> MEKETGPEVDDSKVTYDTIQSKVLKAVIDQAFPRVKEYSLNGHTLPGQVQQFNQVFINNHRITPEVTYKKINETTAEYLMKLRDDAHLINAEMTVRLQVVDNQLHFDVTKIVNHNQVTPGQKIDDESKLLSSISFLGNALVSVSSDQTGAKFDGATMSNNTHVSGDDHIDVTNPMKDLAKGYMYGFVSTDKLAAGVWSNSQNSYGGGSNDWTRLTAYKETVGNANYVGIHSSEWQWEKAYKGIVFPEYTKELPSAKVVITEDANADKNVDWQDGAIAYRSIMNNPQGWEKVKDITAYRIAMNFGSQAQNPFLMTLDGIKKINLHTDGLGQGVLLKGYGSEGHDSGHLNYADIGKRIGGVEDFKTLIEKAKKYGAHLGIHVNASETYPESKYFNEKILRKNPDGSYSYGWNWLDQGINIDAAYDLAHGRLARWEDLKKKLGDGLDFIYVDVWGNGQSGDNGAWATHVLAKEINKQGWRFAIEWGHGGEYDSTFHHWAADLTYGGYTNKGINSAITRFIRNHQKDAWVGDYRSYGGAANYPLLGGYSMKDFEGWQGRSDYNGYVTNLFAHDVMTKYFQHFTVSKWENGTPVTMTDNGSTYKWTPEMRVELVDADNNKVVVTRKSNDVNSPQYRERTVTLNGRVIQDGSAYLTPWNWDANGKKLSTDKEKMYYFNTQAGATTWTLPSDWAKSKVYLYKLTDQGKTEEQELTVKDGKITLDLLANQPYVLYRSKQTNPEMSWSEGMHIYDQGFNSGTLKHWTISGDASKAEIVKSQGANDMLRIQGNKEKVSLTQKLTGLKPNTKYAVYVGVDNRSNAKASITVNTGEKEVTTYTNKSLALNYVKAYAHNTRRNNATVDDTSYFQNMYAFFTTGADVSNVTLTLSREAGDEATYFDEIRTFENNSSMYGDKHDTGKGTFKQDFENVAQGIFPFVVGGVEGVEDNRTH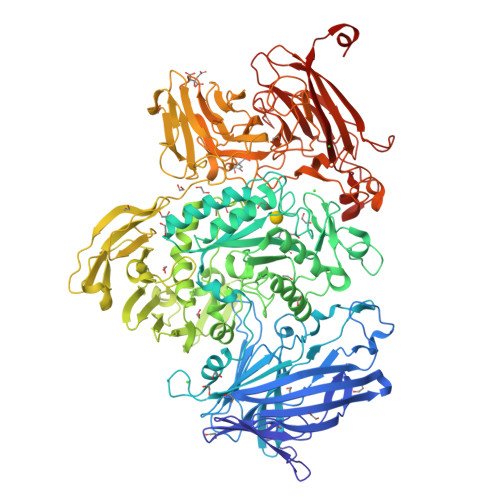LSEKHDPYTQRGWNGKKVDDVIEGNWSLKTNGLVSRRNLVYQTIPQNFRFEAGKTYRVTFEYEAGSDNTYAFVVGKGEFQSGRRGTQASNLEMHELPNTWTDSKKAKKATFLVTGAETGDTWVGIYSTGNASNTRGDSGGNANFRGYNDFMMDNLQIEEITLTGKMLTEHHHHH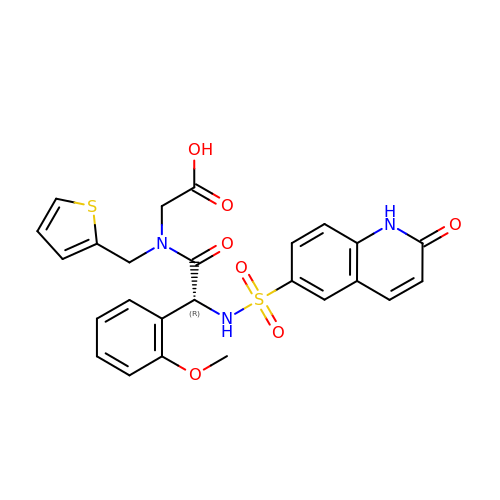N-[(2R)-2-(2-methoxyphenyl)-2-{[(2-oxo-1,2-dihydroquinolin-6-yl)sulfonyl]amino}acetyl]-N-[(thiophen-2-yl)methyl]glycine | C25 H23 N3 O7 S2 | OIUMFGYEVQJCBR-XMMPIXPASA-N N-[[4-(6-methyl-1,3-benzoxazol-2-yl)phenyl]methyl]pyridine-3-carboxamide 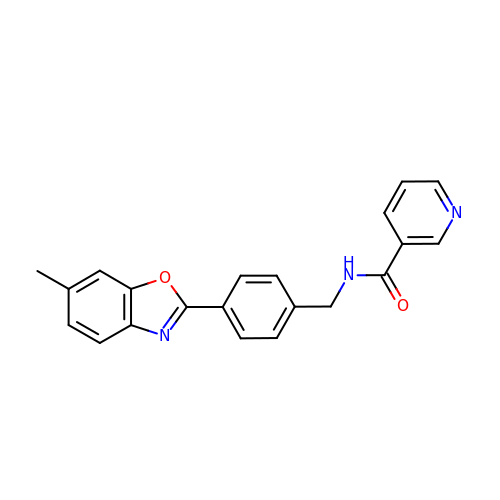| C21 H17 N3 O2 | UNHAWZZVVULEHG-UHFFFAOYSA-N>MGAAPDSHQLAKALAEAADVGAQMIKLVGLRELSEAERQ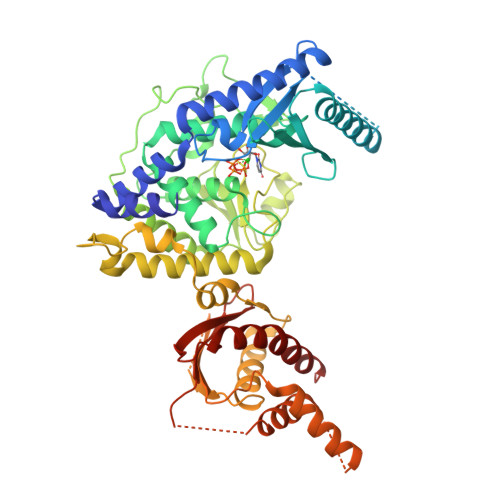LRSLVVALMQEVFTEFFPGCVVHPFGSSINSFDVHGCDLDLFLDLGDLEEPQPVPKLPPASPLLEDREEGDLGKASELAETPKEEKAEGAAMLELVGSILRGCVPGVYRVQTVPSARRPVVKFAHRPSGLHGDVSLSNRLALHNSRFLSLCSELDGRVRPLVYTLRAWAQGRGLSGSGPLLSNYALTLLVIYFLQTRDPPVLPTVSQLTQKAGEGEQVEVDGWDCSFPRDASRLEPSINVEPLSSLLAQFFSAVSSWDLRGSLLSLREGQALPVAGGLPSNLWEGLRLGPLNLQDPFDLSHNVAANVTSRVAGRLQNCCRAAANYCRSLQYQRRSSRGRDWGLLPLLQPSSPSSLLSATPIPLPLAPFTQLTAALVQVFREALGCHIEQATKRTRSEGGGTGQGEAGKGASLPSSASWRCALWHRVWQGRRRARRRLQQQTKEGAGGGAGTRAGWLATEAQVTQELKGLSGGEERPETEPLLSFVASVSPADRMLTVTPLQDPQGLFPDLHHFLQVFLPQAIRHLKLEHHHHHH[2x]> GRSLELGAADIQDLESFEAGRGALPARAYLQSDAPRLSLNGEWQFRLSPGSRVAPDDGWQLGEALNGFESLPVPSSWPMHGHGAPAYTNVQFPFAVEPPHVPEANPIGDHLVVFEAGPEFFPHALLRFDGIESAGTVWLNGVELGTTRGSRLAHEFDVSGILEQGENTLAVRVAQFSAASYVEDQDMWWLPGIFRDVTLQARPAAGIDDVFVHAGYDHITGEGILKVEASRGGQAIDAVVRVPELALELAAGTEVRVPAVEPWSAEVPKLYEAAVSAAGESVALQIGFRSIAIEDAQFKVNGRRILLRGVNRHEHHPRLGRVVPRDVVEAELRLMKQHNINAIRTSHYPPHPQFLALADQLGFYVVLECDLETHGFESAGWAQNPSDDPQWEDALVDRMRRTVERDKNHASVVMWSLGNEAGTGRNLAAMSRWTKDRDPSRPIHYEGDWSSEHVDVYSRMYASQAETALIGQGIEPALNDAALDARRRAMPFVLCEYVHAMGNGPGGMSEYQALF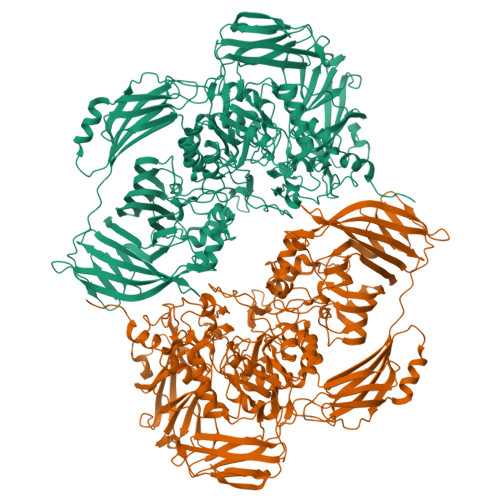EKYPRLMGGFVWEWLEHGITVSTADGVDHYGYGGDFGEEVHDGNFVTDGLVDADRRPRPGLLDFKKVIEPLRIDVARDWTGFTLRNGQDFADTSAFSFRYEVEADGGALDGGTVDVAPVAPQSETVVELPGSVAALAAGLSDGRPAVLTVRAVLGADSAWADAGHEVAWGQSVREPGAPVPPAPVEPVQVQDSELTLGPVVFSRATGMPTSIGGVPVEKLGLTLWWAPTDNDLGREWGGADERPLATQWKDAGLNRLHTRLLGISANPGQDGGETLTVRTRVSAADKQYGVLVDYTWSTDGETVGLRTQVRRDGTWVNRGFEVEWARIGLEFVLGEETELVSWFGQGPHQSYPDTGQGARAGWFSLPLAKMDVEYVRPQECGARSGSRSAALQLGGRTLEICGDPFALTVRPYSQDVLDAAAHRPDLKADGRTYLYVDHALRGVGTAACGPGVLEQYRLKPRDADFILTLKVRS>[4x]FEEEDVICDGCNGPVVGTRYKCSVC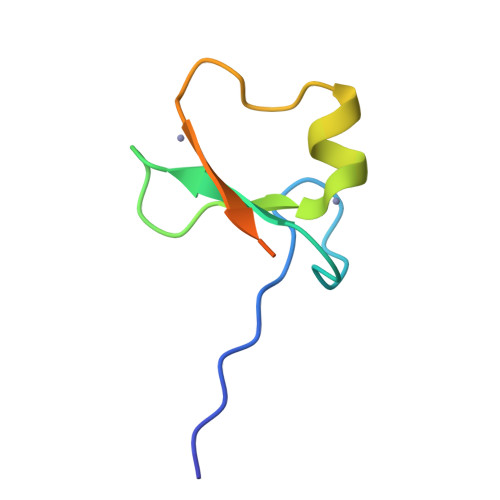PDYDLCSVCEGKGLHRGHTKLAFPSPFGHLSEGFS> MSDPLHVTFVCTGNICRSPMAEKMFAQQLRHRGLGDAVRVTSAGTGNWHVGSCADERAAGVLRAHGYPTDHRAAQVGTEHLAADLLVALDRNHARLLR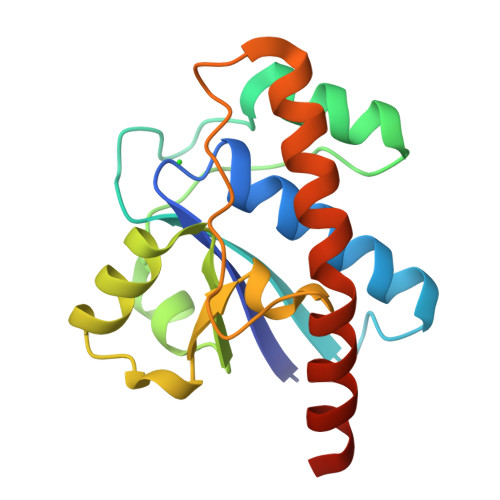QLGVEAARVRMLRSFDPRSGTHALDVEDPYYGDHSDFEEVFAVIESALPGLHDWVDERLARNGPS>[2x]MGSSHHHHHHSSGRENLYFQGMNTLQLINKNHPLKKNQEPPHLVLAPFSDHDVYLQPEVAKQWERLVRATGLEKDIRLVSGYRTEKEQRRLWEYSLKENGLAYTKQFVALP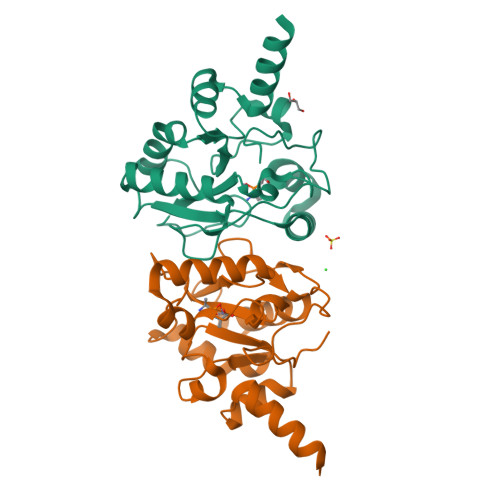GCSEHQIGLAIDVGLKKQEDDDLICPHFRDSAAADLFMQQMMNYGFILRYPEDKQEITGISYEPWHFRYVGLPHSQVITAQKWTLEEYHDYLAQTVRQFA>MAYRDQPLGELALSIPRASALFRKYDMDYAAGGKQTLARAAARKELDVEVIEAELAKLAEQPIEKDWRSAPLAEIIDHIIVRYHDRHREQLPELILQATKVERVHADKPSVPKGLTKYLTMLHEELSSHMMKEEQILFPMIKQGMGSQAMGPISVMESEHDEAGELLEVIKHTTNNVTPPPEACTTWKAMYNGINELIDDLMDHISLENNVLFPRAL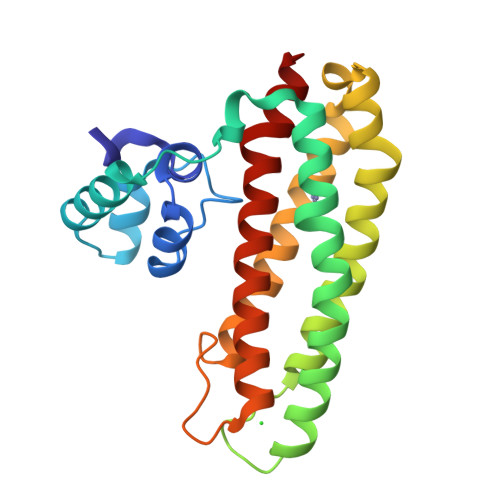AGE[2x]>[6x]MVRLGPKKPPARKGSMADVPANLMEQIHGLETLFTVSSEKMRSIVKHFISELDKGLSKKGGNIPMIPGWVVEYPTGKETGDFLALDLGGTNLRVVLVKLGGNHDFDTTQNKYRLPDHLRTGTSEQLWSFIAKCLKEFVDEWYP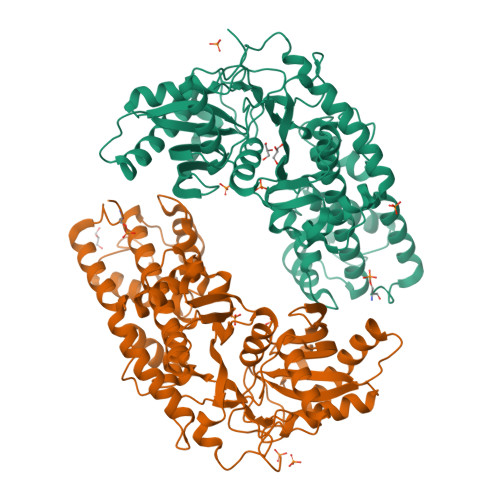DGVSEPLPLGFTFSYPASQKKINSGVLQRWTKGFDIEGVEGHDVVPMLQEQIEKLNIPINVVALINDTTGTLVASLYTDPQTKMGIIIGTGVNGAYYDVVSGIEKLEGLLPEDIGPDSPMAINCEYGSFDNEHLVLPRTKYDVIIDEESPRPGQQAFEKMTSGYYLGEIMRLVLLDLYDSGFIFKDQDISKLKEAYVMDTSYPSKIEDDPFENLEDTDDLFKTNLNIETTVVERKLIRKLAELVGTRAARLTVCGVSAICDKRGYKTAHIAADGSVFNRYPGYKEKAAQALKDIYNWDVEKMEDHPIQLVAAEDGSGVGAAIIACLTQKRLAAGKSVGIKGE> VEWTDQERATISSIFGSLDYDDIGPKALSRCLIVYPWTQRHFGSFGNLYNAEAIIGNQKVAAHGIKVLHGLDRAVKNMDNIKEIYAELSILHSEKLHVDPDNFKLLADCLTIVVAAKMGSGFNPGTQATFQKFLAVVVSA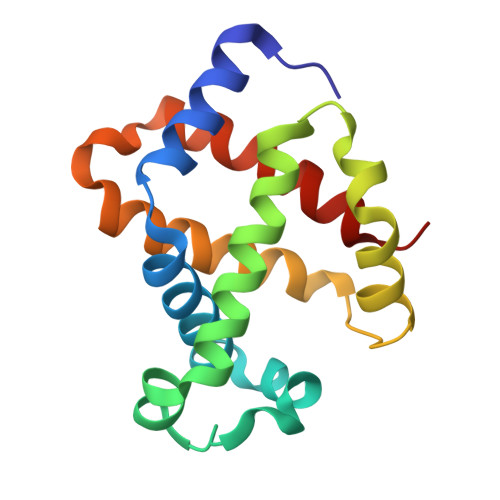LGKQYH(2E)-3-phenylprop-2-enal | C9 H8 O | 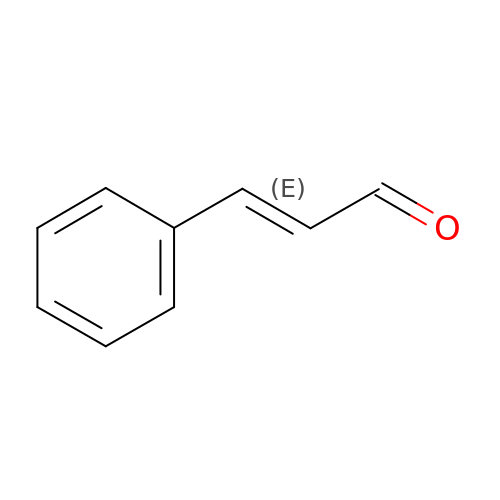KJPRLNWUNMBNBZ-QPJJXVBHSA-N>GAMNAQAEEFKKYLETNGIKPKQFHKKELIFNQWDPQEYCIFLYDGITKLTSISENGTIMNLQYYKGAFVIMSGFIDTETSVGYYNLEVISEQATAYVIKINELKELLSKNLTHFFYVFQTLQKQVSYSLAKFNDFSINGKHGSICGQLLILTYVYGKETPDGIKITLDNLTMQELGYSSGIAHSSAVSRIISKLKQEKVIVYKNSCFYVQNLDYLKRYAPKLDEWFYLACP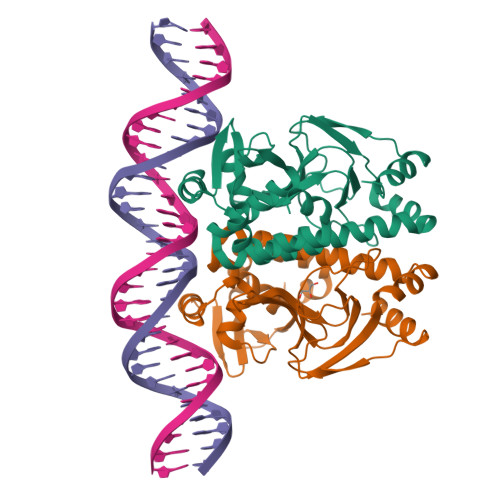ATWGKLN[2x]> DRHHHHHHKLQHAPPWTEDCRKSTYPPSGPTYRGAVPWYTINLDLPPY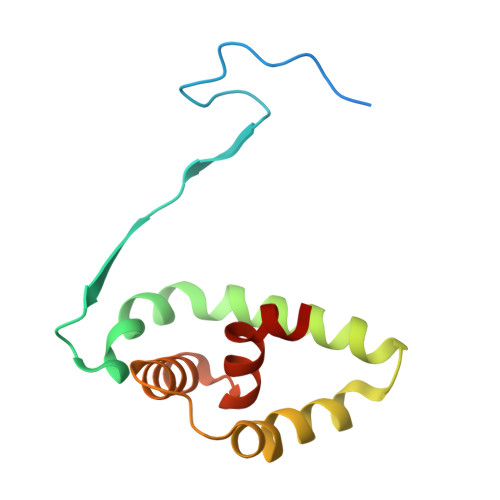KRWHELMLDKAPMLKVIVNSLKNMINTFVPSGKVMQVVDEKLPGLLGNFPGPFEEEMKGIAAVTDIPLGEIISFNIFYELFTI GUANOSINE-P3-ADENOSINE-5',5'-TRIPHOSPHATE | C20 H27 N10 O17 P3 | 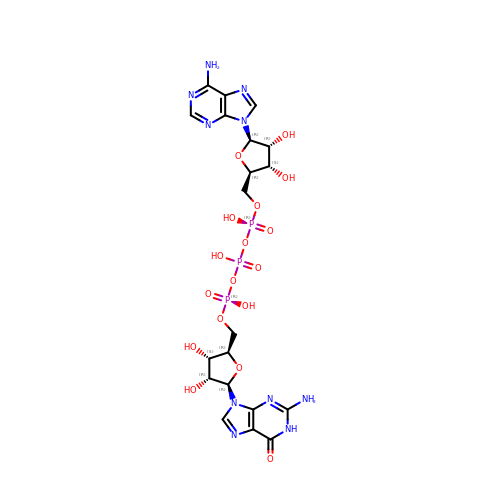PMJUJCUPNRCBNP-INFSMZHSSA-N> XL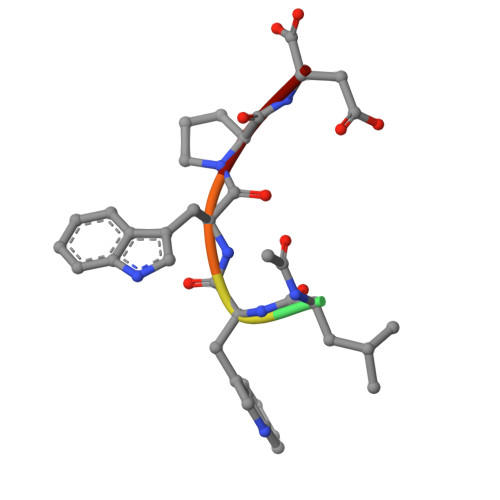WWPD We describe here the use of an artificial cofactor employing the well‐known biotin‐streptavidin system to catalyze a Baylis‐Hillman reaction. As protein host, we chose streptavidin, as it can be easily crystallized and thereby supports the design process. There are several examples using streptavidin as the host for these cofactors, since its natural ligand biotin binds strongly (K d∼10−15 M) and is easy to modify with catalysts at the carboxylic acid group. No enzyme is known to naturally catalyze the Baylis‐Hillman reaction, a very versatile and atom‐economic C−C bond forming reaction for the production of various functionalized compounds and intermediates of active pharmaceutical ingredients (APIs).

We chose a derivative of DMAP as the artificial cofactor due to its low steric demand, which will facilitate its inclusion into the protein scaffold. The protein host around the cofactor was rationally designed on the basis of high‐resolution crystal structures obtained after each variation of the amino acid sequence. The location of the catalyst is in a shallow cavity at the surface of the protein. The system was evolved through repeated cycles of mutagenesis, activity tests, and structure determination. According to the presented structures and calculations the catalytically active site is too shallow to undergo interactions with 1.

>MASMTGGQQMGRREAGITGTWYNQLGSTFIVTAGADGALTGTYESAAGKAESRYVLTGRYDSAPATDGSGTALGWTVAWKNNYRNAHSATTWSGQYVGGAEARINTQWLLTFGATEANGWASTYVGHDTFTKVKPSAASIDAAKKAGVNNGNPLDAVQQ[2x]>[8x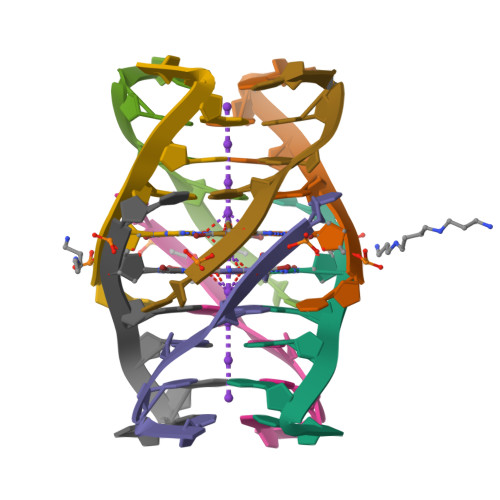]UGAGGU> MSNPIRDIQDRLKTAKFDNKDDMMNLASSLYKYEKQLMDSSEATLCQQGLSNRPNSFSQLSQFRDSDIQSKAGGQTGKFWQNEYEACKNFQTHKERRETLEQIIRFLQNGAEEKDADDLLLKTLARAYFHRGLLYRPKGFSVPARKVEAMKKAIAYCEIILDKNEEESEALRIWLYAAMELRRCGEEYPENFAEKLFYLANDGFISELYDIRLFLEYTEREEDNNFLDMILQENQDRERLFELCLYKARACFHLNQLNDVRIYGESAIDNAPGAFADPFWDELVEFIRMLRNKKSELWKEIAIKAWDKCREKEMKVGNNIYLSWYWARQRELYDLAFMAQDGIEKKTRIADSLKSRTTLRIQELNELRKDAHRKQNRRLEDKLDRIIEQENEARDGAYLRRNPPCFTGGKREEIPFARLPQNWIAVHFYLNELESHEGGKGGHALIYDPQKAEKDQWQDKSFDYKELHRKFLEWQENYILNEEGSADFLVTLCREIEKAMPFLFKSEVIPEDRPVLWIPHGFLHRLPLHAAMKSGNNSNI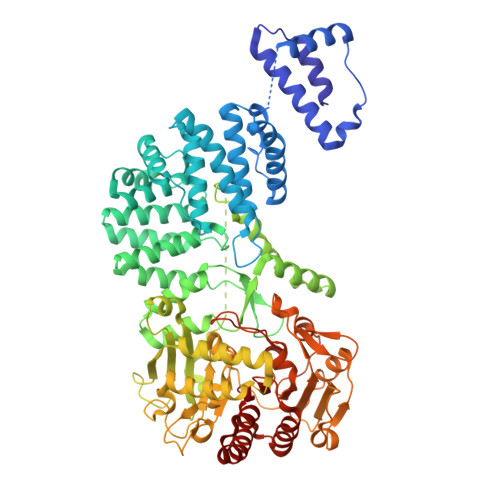EIFWERHASRYLPAWHLFDPAPYSREESSTLLKNFEEYDFQNLENGEIEVYAPSSPKKVKEAIRENPAILLLLCHGEADMTNPFRSCLKLKNKDMTIFDLLTVEDVRLSGSRILLGACESDMVPPLEFSVDEHLSVSGAFLSHKAGEIVAGLWTVDSEKVDECYSYLVEEKDFLRNLQEWQMAETENFRSENDSSLFYKIAPFRIIGFPAE>GSHMDSTTIQQNKDTLSQIVVFPTGNYDKNEANAMVNRLANIDGKYLNALKQNNLKIKLLSGKLTDEKEYAYLKGVVPKGFEGTGKTWDDVPGLGGSTVALRIGFSNKGKGHDAINLELHETAHAIDHIVL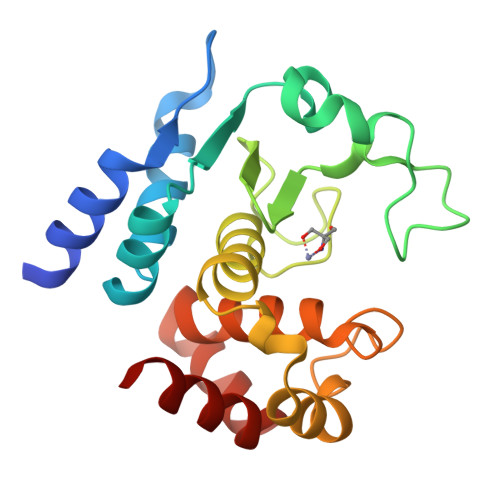NDISKSAQFKQIFAKEGRSLGNVNYLGVYPEEFFAESFAYYYLNQDTNSKLKSACPQTYSFLQNLAK[2x]>[2x]GMTFEPYPFERLRALLKEITPKKRGLDLGIGEPQFETPKFIQDALKNHTHSLNIYPKSAFEESLRAAQRGFFKRRFKIELKENELISTLGSREVLFNFPSFVLFDYQNPTIAYPNPFYQIYEGAAKFIKAKSLLMPLTKENDFTPSLNEKELQEVDLVILNSPNNPTGRTLSLEELISWVKLALKHDFILINDECYSEIYENTPPPSLLEACMLAGNEAFKNVLVIHSL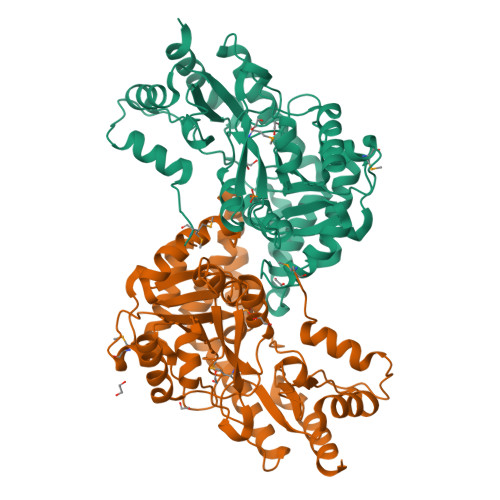SKRSSAPGLRSGFIAGDSRLLEKYKAFRAYLGYTSANAIQKASEAAWLDDRHAEFFRNIYANNLKLARKIFKNTLIYPYSFYVYLPVQNGENFAKTLYQNEGIITLPALYLGRNRIGADYVRLALVYDTPLLEKPLEIIETYRENHA> MSLRPRVLLVE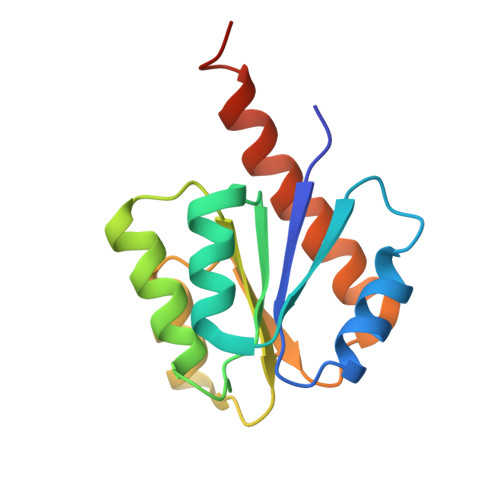DSTSLAILYKQYVKDEPYDIFHVETGRDAIQFIERSKPQLIILDLKLPDMSGEDVLDWINQNDIPTSVIIATAHGSVDLAVNLIQKGAEDFLEKPINADRLKTSVALHLKRAKLEDLVEGHHHHHH>[6x]MAYQYVNVVTINKVAVIEFNYGRKLNALSKVFIDDLMQALSDLNRPEIRCIILRAPSGSKVFSAGHDIHELPSGGRDPLSYDDPLRQITRMIQKFPKPIISMVEGSVWGGAFEMIMSSDLIIAASTSTFSMTPVNLGVPYNLVGIHNLTRDAGFHIVKELIFTASPITAQRALAVGILNHVVEVEELEDFTLQMAHHISEKAP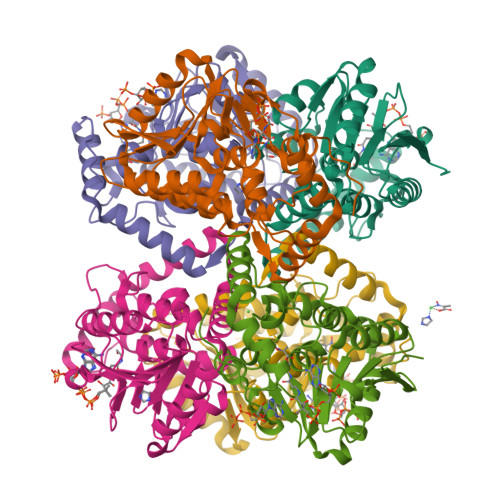LAIAVIKEELRVLGEAHTMNSDEFERIQGMRRAVYDSEDYQEGMNAFLEKRKPNFVGH> FQSSAMVLRDGAKFEAQAGDPTQALETYKDAMVASGVTTTRPQDNDTFTRLTRNDEKDDWLKRGVRSDAADLYRQQDLNVTLEHDYWGSSGTGGYSDLKAHTTMLQVDAPYSDGRMFFRSDFVNMNVGSFSTNADGKWDDNWGTCTLQDCSGNRSQSDSGASVAVGWRNDVWSWDIGTTPMGFNVVDVVGGISYSDDIGPLGYTVNAHRRPISSSLLAFGGQKDSPSNTGKKWGGVRADGVGLSLSYDKGEANGVWASLSGDQLTGKNVEDNWRVRWMTGYYYKVINQNNRRVTIGLNNMIWHYDKDLSGYSLGQGGYYSPQEYLSFAIPVMWRERTENWSWELGASGSWSHSRTKTMPRYPLMNLIPTDWQEEAARQSNDGGSSQGFGYTARALLERRVTSNWFVGTAIDIQQAKDYAPS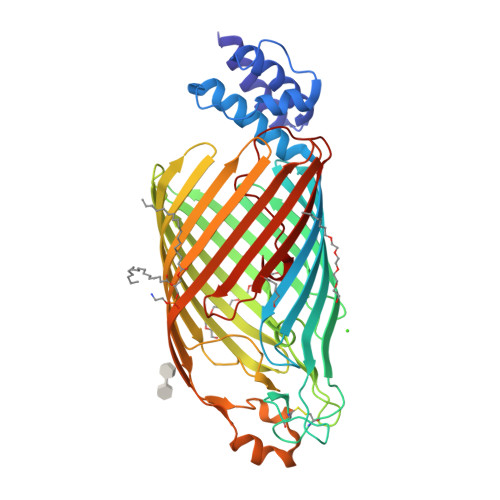HFLLYVRYSAAGWQGDMDLPPQPLIPYADW2-[5-ethyl-2,4,6-tris(oxidanylidene)-1,3-diazinan-5-yl]ethyl selenocyanate | C9 H11 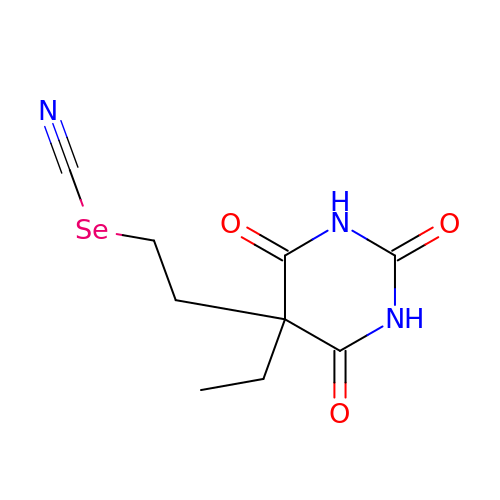N3 O3 Se | LFTCFIKEJOPJTJ-UHFFFAOYSA-N> GPLGSGIPMFLEKINQKTGEREWVVAEEDYDMAQELARSRFGDMILDFDRNDKFLAGLKTTIAEKKHENTDGKVHVLDIGTGTGLLSLMAAREGADKVTALEVFKPMGDCARHITSNSPWSDKITVISERSTDVSQIGGSRADIIVAEVFDTELIGEGALRTFKEALERLAKPGCRVVPSTGNVYIVPVESHLLKMFNDIPRLNGEKDEEPLGRCSGTAAVFDVQLSEMKTHEFRELSEPIVAFKFDFEHEEKIIFDESFVREAVAHSSGTIDALLMWWDIDMDRNGTTFIDMGPKWKNKNNYAWRDHWMQAVYYLPEKKKVEMNQTFEIVCNHDEFSLWFSNVGKDKSRSYCVCGLHSMLSRQTVYHVNEMFENQKFKDEVDKLSKGLHVATVGEGSFLGLLAAKTAKRVTIIDGNERFRDIFFKYIHYYKLTNVEIIEKVTSLTDSPDIVLAEPFYMSAMNPWNHLRFLYDVEVLKMMHGDELRVEPHMGVLKAIPEKFEDLQNIASDVGTVNGFDLSFFDEISTKARTA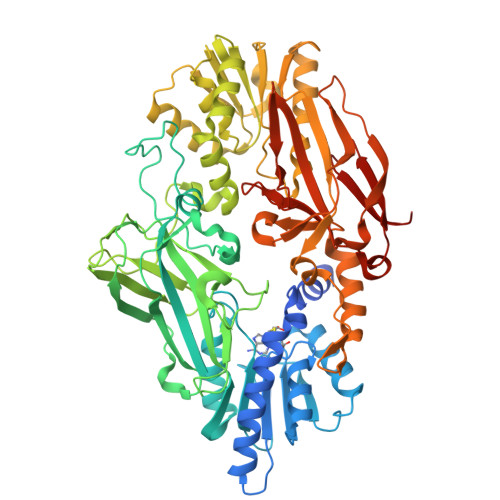TDAIVDEQSLWEYAGIVKGDAVEILRFPIDGRVSSQKCVVNIDNMSSSNAIPMWMEWEFGGINLSTGLLSISSAGVPEWNKGYKQGVYFPITALRNDKSLCLHALFDKSTGDINFQFGKSEDS We have determined the crystal structures of DNA duplexes containing -CGCCG- regions as CCG repeat motifs that comprise a non-CpG site with or without cytosine methylation. On the other hand, methylation of cytosines immediately preceding a non-guanine residue is known as non-CpG methylation. Our structural results demonstrated that cytosine methylation at a non-CpG step leads to an anti→syntransition of its complementary guanosine residue toward the (w)cWH geometry as a partial population of WC, in both drug-bound and naked mC:G base pairs. This particular geometry is specific to non-CpG methylated dinucleotide sites in B-form DNA.

To further test whether base pair dynamics are primarily responsible for the polymorphic base pair geometry that promote (w)cWH formation, we replaced the guanine of the center mC:G pair with inosine. Since the only difference between guanine and inosine is the absence of the N2 amino group in inosine, this substitution is ideal for reflecting the base pair instability associated with the loss of a single H-bond. The unliganded C:I pairing structure was determined at a resolution of 2.5 Å. Each asymmetric unit contains four independent duplexes, labelled C:I-NPX1 to C:I-NPX4. The central C4:I11 base pairs in all four duplexes adopt a single anti–antipair in a non-canonical WC geometry. This could be attributed to the instability of WC pairing due to the loss of H-bonds. However, we did not observe any alternative conformations in C:I-NPXs. Our results showed that higher fluctuation was observed at the central bases of the C:I-NPX1 compared to the native unmethylated structure. This indicates that substitution of guanine by inosine enhanced base pair dynamics. Using the unmethylated sequence, we introduced additional base pair instability by substituting the guanosine with an inosine, which results in the loss of an H-bond, leading to only a single base pair geometry in the structure, even though the dynamics of the C:I base pair had been enhanced compared to the original sequence.

>[4x]ACGCCGT;>ACGICGT[4x]> MSGILDRCTCTPNARVFVAEGQVYCTRCLSARSLLPLNLQVPELGVLGLFYRPEEPLRWTLPRAFPTVECSPA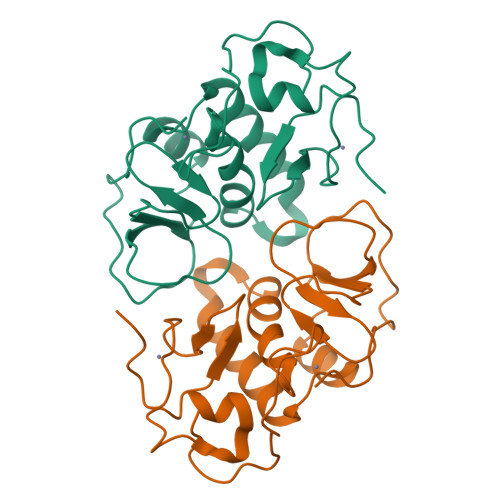GACWLSAIFPIARMTSGNLNFQQRMVRVAAEIYRAGQLTPTVLKTLQVYERGCRWYPIVGPVPGVGVYANSLHVSDKPFPGATHVLTNLPLPQRPKPEDFCPFECAM> GTSTQTKAGSLTIVGTGIESIGQMTLQALSYIEAAAKVFYCVID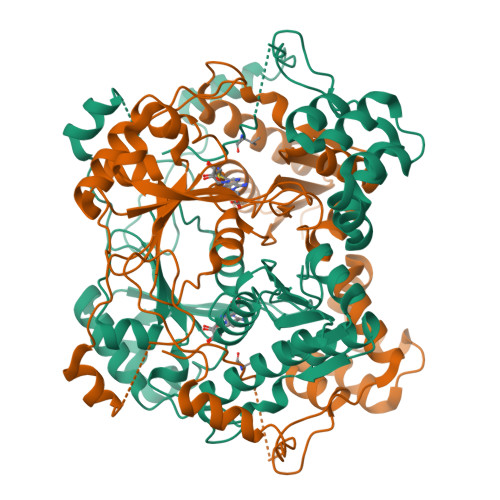PATEAFILTKNKNCVDLFQYYDNGKSRLNTYTQMSELMVREVRKGLDVVGVFYGHPGVFVNPSHRALAIAKSEGYRARMLPGVSAEDCLFADLCIDPSNPGCLTYEASDFLIRDRPVSIHSHLVLFQVGCVGIADFNFTGFDNNKFGVLVDRLEQEYGAEHPVVHYIAAMMPHQDPVTDKYTVAQLREPEIAKRVGGVSTFYIPPKARKASNLDIIRRLELLPAGQVPDKKARIYPANQWEPDVPEVEPYRPSDQAAIAQLADHAPPEQYQPLATSKAMSDVMTKLALDPKALADYKADHRAFAQSVPDLTPQERAALELGDSWAIRCAMKNMPSSLLDAARESGEEASQNGFPWVIVVGVIGVIG> GSHMNNRVVKLAAGSNTQTVLPFTGLNTPSGVAVDSAGTVWVTDHGNNRVVKLAAGSNTQTVLPFTGLNTPSGVAVDSAGTVWVTDHGNNRVVKLAAGS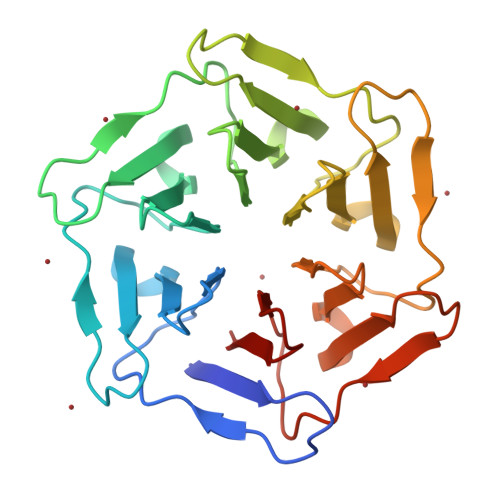NTQTVLPFTGLNTPSGVAVDSAGTVWVTDHGNNRVVKLAAGSNTQTVLPFTGLNTPSGVAVDSAGTVWVTDHGNNRVVKLAAGSNTQTVLPFTGLNTPSGVAVDSAGTVWVTDHGNNRVVKLAAGSNTQTVLPFTGLNTPSGVAVDSAGTVWVTDH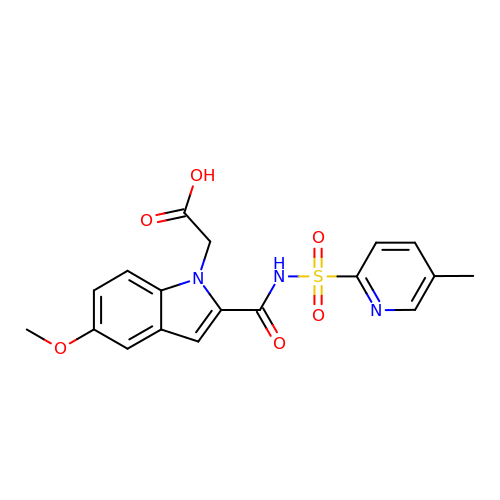(5-methoxy-2-{[(5-methylpyridin-2-yl)sulfonyl]carbamoyl}-1H-indol-1-yl)acetic acid | C18 H17 N3 O6 S | MOZJRLFDFCKFFT-UHFFFAOYSA-N> MNGSADAGPRPRKYVFITGGVVSSLGKGILTSSLGALLRARGYRVTAIKIDPYVNVDAGTMRPYEHGEVFVTADGAETDLDIGHYERFLDMDLSRGNNLTTGQVYLSVIQKERRGEYLSQTVQVIPHITDEIKERIRKVAEEQKAEIVVVEVGGTVGDIESLPFLEAIRQFRFDEGEGNTLYLHLTLVPYLETSEEFKTKPTQHSVATLRGVGIQPDILVLRSARPVPEEVRRKVALFTNVRPGHVFSSPTVEHLYEVPLLLEEQGLGRAVERALGLEAVIPNLSFWQEAVRVLKHPERTVKIAIAGKYVKMPDAYLSLLEALRHAGIKNRARVEVKWVDAESLEAADLDEAFRDVSGILVPGGFGVRGIEGKVRAAQYARERKIPYLGICLGLQIAVIEFARNVAGLKGANSTEFDPHTPHPVI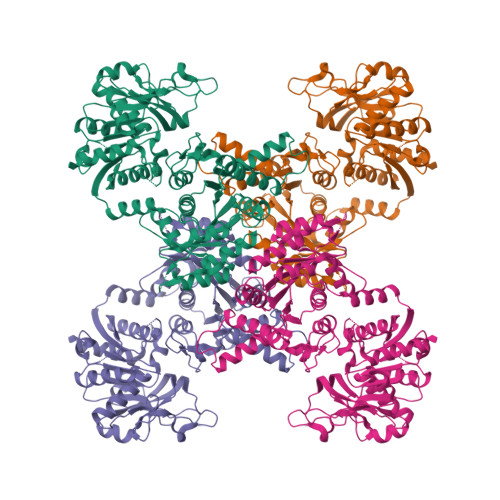DLMPEQLEVEGLGGTMRLGDWPMRIKPGTLLHRLYGKEEVLERHRHRYEVNPLYVDGLERAGLVVSATTPGMRGRGAGLVEAIELKDHPFFLGLQSHPEFKSRPMRPSPPFVGFVEAALAYQERA> MSSVIREIAKRFLEQATINIAEEVVREYGDHERTMISVGVHFQACCLISDEYTLEDETTPRYVLLEGLKRQEAISKQNNICSTLGLEPLRNLADIFDRKTRRFLEVGITKRESDEYYQEKFNKIGNDMDIHVFTYEGKYFSNNPNGLEDIQKTRIFTFLSFVSDELRKENMFTEMYVTEEGAPELEMYKSKLFIAMRDESVPLPYINYEHLRTRCETFKRNQAECEAKVADVASRLKIKLEHLEENKLRPLEIPKEKEAPYTHKFLMKDAWFFAKPHDSERAQPQQILYDFFEAANMGFMTTSPKPIFGKQGLMYHSLWGQTKRAIKDKRNELEPSEQRDFLCGIGRASKKIQEDKWQESREEEFKQEETKGAAKRGFPTWFNEEWLWAMRDSGDGDNKIGDWIPMAEMPPCKNEMEDYAKKMCEELESKIQGTNCAREMSKLIHTIGSLHTECRNFPGKVKIVPIYCRGTLRGESTDCLFGIAIKGKSHLNKDDGMYTVVTFEFSTEEPNPSKHEKYTVFEAGTVPVEAVVLTPKRERVLKEKKLFLYCRTTGMSKLKNDWFSKCRRCLIPTMETVEQIVLKECAL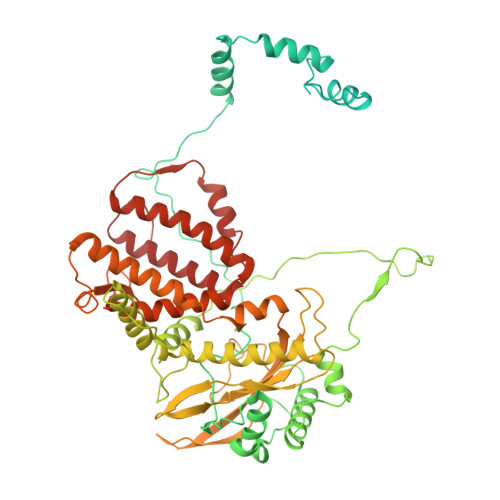KEENRVSEMLENKRAWIAHENGENLTRLVSTKLKDLCRMLIVTQFYYCIYNDNQLEGFCNEQKKFLMFLQADKDSKSAFTFNQKGLYEKIEECIVSNPLCIFLADRLNKLFLVAKSNGAKYFE>GNKLFNIAQRILDTNSVLLTERGDHIVWINNSWKFNSEEPLITKLILSIRHQLPKEYSSELLCPRKRKTVEANIRDMLVDSVETDTYPDKLPFKNGVLDLVDGMFYSGDDAKKYTCTVSTGFKFDDTKFVEDSPEMEELMNIINDIQPLTDENKKNRELYEKTLSSCLCGATKGCLTFFFGETATGKSTTKRLLKSAIGDLFVETGQTILTDVLDKGPNPFIANMHLKRSVFCSELPDFACSGSKKIRSDNIKKLTEPCVIGRPCFSNKINNRNHATIIIDTNYKPVFDRIDNALMRRIAVVRFRTHFSQPSGREAAENNDAYDKVKLLDEGLDGKIQNNRYRFAFLYLLVKWYKKYHIPIMKLYPTPEEIPDFAFYLKIGTLLVSSSVKHIPLMTDLSKKGYILYDNVVTLPLTTFQQKISKYFNSRLFGHDIESFINRHKKFANVSDEYLQYIFIEDISSP[6x]

Helicase E5 is a multi-domain protein; its primer synthesis and DNA unwinding activity are required for genome uncoating and DNA replication of MPXV. MPXV E5 is encoded by the E5R gene, the mature protein is 785 amino acids (aa) in length. MPXV E5 can be divided into 6 domains: the AEP domain, the ZnD domain (Zinc-binding domain), the D5N domain (a domain associated with D5-type helicases), the Linker, the SF3 Helicase domain, and the C-Tail. MPXV E5 belongs to the SF3 helicase superfamily, which normally forms hexamer and unwinds DNA with 3′- to 5′ polarity.

To this end, we constructed and purified one MPXV E5 protein (aa 322–785) with N-terminus truncated, which is termed as E5_∆N hereafter. As shown by in vitro DNA unwinding assays, E5_∆N has no unwinding activity towards DNA (50 nM) with T15 at either 5′- or 3′-overhang region, but the forked DNA can be efficiently unwound by E5_∆N. About 60% of forked DNA is unwound by E5_∆N with a concentration of 50 nM. Like the E5-ssDNA-AMPPNP complex, the 6-nt ssDNA fragment was captured by the SF3 helicase domains of monomers A to D in the E5_∆N-ssDNA-AMPPNP structure. Structural superposition shows that the conformations of the DNA and the four DNA-interacting SF3 helicase domains are virtually identical in the two complex structures, indicating that truncation of the N-terminus does not alter the DNA-binding mode by MPXV E5. Compared to the E5-ssDNA-AMPPNP structure, the overall resolution of the E5_∆N-ssDNA-AMPPNP structure is higher (2.67 Å). Three AMPPNP molecules were captured in the E5_∆N-ssDNA-AMPPNP structure, associated with the SF3 domains of monomers A, B, and C, respectively; the conformations of the AMPPNPs are identical to these in the E5-ssDNA-AMPPNP structure. No AMPPNP was associated with the monomers D and F in the E5_∆N-ssDNA-AMPPNP structure; their ATP-interacting loops are disordered. Compared with the E5-ssDNA-AMPPNP structure, the gap between the SF3 helicase domains of monomers F and A is wider; in addition, the helicase domain of monomer E is completely disordered in the E5_∆N-ssDNA-AMPPNP structure. In the E5_∆N-ssDNA-AMPPNP structure, only one C-Tail (of monomer A) was observed.>[2x]MSQEQYTENLKVIVAEKLAGIPNFNEDIKYVAEYIVLLIVNGGT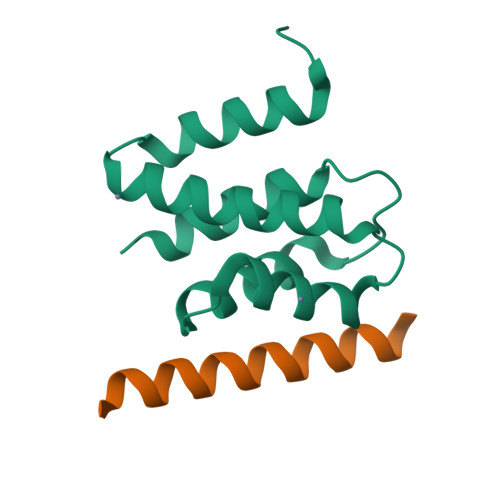VESVVDELASLFDSVSRDTLANVVQTAFFALEALQQGESAENIVSKIRMMNAQSLGQSDIA;>[2x]KQDTASKMKLLKKKIEEQREILQKTHHKN>[4x]GPKLREVKYELDTKVSELSHKLGSSEGSNRSLEEETARLRSLNQQLSSSKHELEIQLNEAKAKVLALDEKAQSQGDVIEQQRGRLRDMEAALRQTEQRCADLRDTLASAEGRAKEA

Centrioles have proximal-distal polarity and a 9-fold radial symmetry imparted by a likewise symmetrical central scaffold, the cartwheel. The spindle assembly abnormal protein 6 (SAS-6) self-assembles into 9-fold radially symmetric ring-shaped oligomers that stack via an unknown mechanism to form the cartwheel. SAS-6 proteins comprise a globular “head” domain at their N-terminus followed by a long coiled coil that mediates stable protein homo-dimerization (Keller et al., 2014), and a disordered C-terminal extension. The characteristic shape of the SAS-6 ring led to the proposal that the protein head domains comprise the central “hub” of the centriolar cartwheel, with SAS-6 coiled coils forming the cartwheel “spokes” (Cottee et al., 2015; Kitagawa et al., 2011; van Breugel et al., 2011; van Breugel et al., 2014; Yoshiba et al., 2019).

In contrast, structures of the CrSAS-6_CCMiddle fragment, resolved from two different crystal forms, revealed parallel complexes featuring extensive interaction interfaces between coiled-coil domains, within each crystal’s asymmetric unit. In CrSAS-6_CCMiddle crystal form I, resolved to 2.34 Å using SeMet-derived experimental phasing two copies of the coiled-coil domain in the asymmetric unit interacted over almost their entire ∼16 nm length. The association was driven primarily via ionic and hydrogen-bonding interactions between CrSAS-6 amino acid side chains, with only a small hydrophobic contribution involving the sidechain of L339, resulting in ∼1,400 Å2 of buried solvent-accessible surface area. In crystallographic structures of the CrSAS-6 coiled coil, we showed that these domains form a unit equivalent to two cartwheel spokes merging together. They do so by associating into a parallel coiled-coil complex, the formation of which does not perturb canonical domain structure; for example, the coiled coils do not unwind or adopt a tetrameric coiled-coil arrangement. Rather, complex formation relies on ionic and hydrogen-bonding interactions interspersed along the length of the coiled coils, and is very weak in solution. We evaluated that an L339E/D378N double mutation of the CrSAS-6 coiled coil (CrSAS-6_CCLD) would have the largest impact on the symmetric interaction mode, as these substitutions remove the sole hydrophobic contact seen in the symmetric complex interface (L339-L339′), as well as two salt bridges of the same complex (D378-R377′ and the symmetry-related pair). In contrast to this prediction, however, reconstitution assays with CrSAS-6LD produced abundant cartwheels, similar to those generated using the corresponding WT protein. We surmised that amino acid substitutions that remove favorable interactions of the symmetric CrSAS-6 coiled-coil complex do not affect cartwheel formation in vitro.> MKLLHERMMHSLARYPRQTAVVDEQDALSYEALELRIREFVAMLCALGVGQGQRILLWAHKSVDLVAVMQAALRLGVVYVPVDPLSPVSRLEKIAGDSQAVLVLCTAARLEELAGSALAQVRSVVLDDPASAGYWRNIDTGSSVVPTLAIQPDDLAYILYTSGSTGVPKGVALSHGNALAFVDWACERYCFQPGERFANHAPLHFDLSVLDIYCALNVGATVCLVPESIAFSPRLLTDFIRQHEISI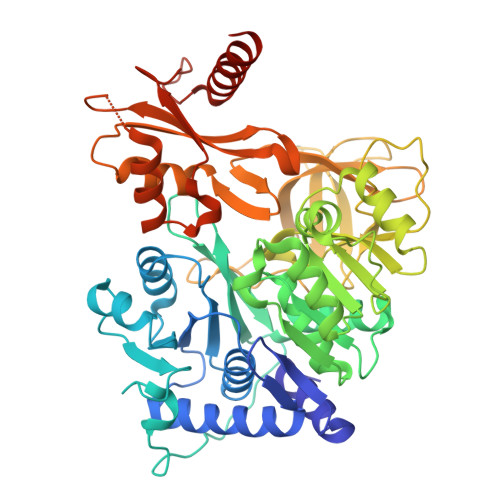WYSVPSVLMMMMQDGDLLSDIQDTLRVLLFAGEPFPVKHLRDLRAAYADVRLANLFGPTETNVCTAFEVGAIDPERVLPVPIGTAASGNQVWAQKPDGSRCAVGEEGELVVQGPTVMLGYFAKPAQEGPYKTGDMVRQRPDGNYEYLGRRDDMLKVRGNRIERGEVEAALLAHPQVSEAAVLVVGEGMNAQLWGVLVAHTRDALSLIDLKRHCAQRLPRYMIIDKVLCLDALPRNANGKVDRFALARQVEGKLAAALEHHHHHHHH> LFSQIELSFSASNLRDRDVLSKSDPMVVVYQKEKDATLSEVFRSEVVLNSLAPKWIKKFIVAYHFETVQTLVFRVYDVDTKFQNSREEMLKLDEQQFLGEATCALSEIITKSTRTSTLELKRKDGFAPQAQPHHGKLIIHAEESLASKISTEIVFRCSNLESKDLFSKSDPFLVVSKIVEHGTPIPVSKTEVRKNDLNPIWKPVFLSVQQVGSKDSPVIIECSDFNSNGKHSLIGKVQKSLSDLEKLHLAGQGINFSLPTGAGQNKVLKSQLFVDKFTETVHHTFLEYLASGFELNFMVAIDFTASNGNPRLPDSLHYIDPSGRLNAYQRAIMDVGEVLQFYDSDKRFPAWGFGARPIDAPVSHCFNLNGSSSYSEVDGIQGIMTSYTS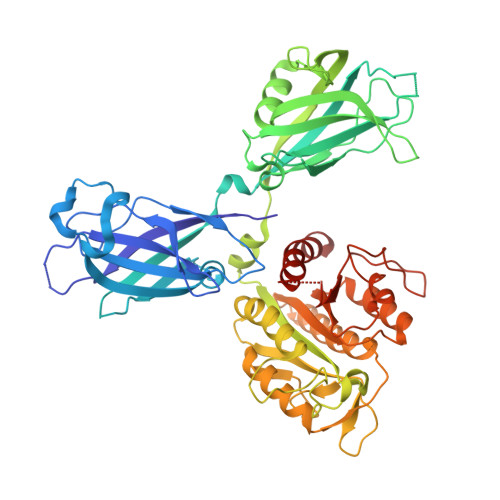ALFNVSLAGPTLFGPVINAAAMIASASLAQGSRKYYVLLIITDGVITDLQETKDALVSASDLPLSILIVGVGGADFKEMEILDADKGERLESSSGRLASRDIVQFVALRDVQYGEISVVQALLAELPSQFLTYMRIR>[2x]ENGEGTTQPDYDNSTDYYNYEDFKCTCPAPHLNNTNGTVMKPIGCYYTCNVTRCTAPDTYPCYNLTEHQAKNLTTSPTTLCAVGNCDHGICVPNGTKELCFKAPNLEE;>GPSQP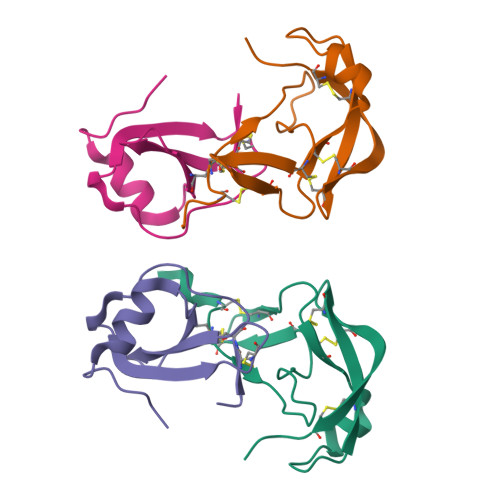KVPEWVNTPSTCCLKYYEKVLPRRLVVGYRKALNCHLPAIIFVTKRNREVCTNPNDDWVQEYIKDPNLPLLPTRNLSTVKIITAKNGQPQLLNSQ[2x]>[14x]MAKELHFNKDMQALKRMQAGVDKLATVVGVTIGPKGRNVVLESKFGAPKIVNDGVTIAREVELSDPVENIGATLVRQAAARTNDTAGDGTTTATVLSAAFIAEGMKIVSAGTNPVQLVRGMEKTVQELVKELRKMSSVVQTDKDLANVACVSAGGNTDIGSLISDAMAKVGRTGVVTMEEGKTAEDQLVFVEGMQFERGYTSPYFVTDPERMICEYENCKILLVDKKISTARDIITILESAIRGNYPLLIMAEEVEQEALATLVVNKLRGTLKVVAIKAPGFGERRSSYLEDIAILTGGTV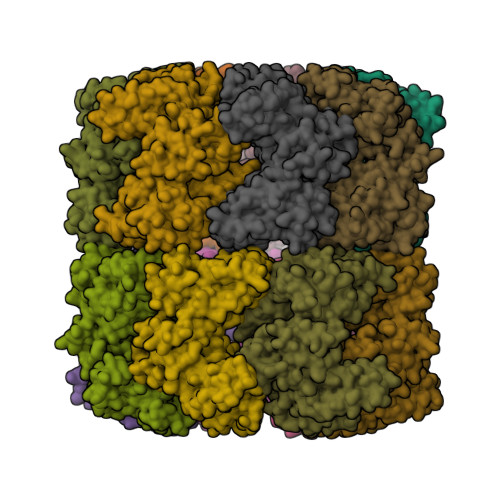VRDEMGVSLEQATDAVLGTAAKITITKERTTVVGDGSTAADVAARVKQIRNLQMQTDQDYEREKLQERIARLSGGVAIIQVGAQTETELKEKKLRVEDALNATRAAVEEGVVPGGGCTLLRLSEKVDVIKRRMTDPEQQMGADIIKRALCYPIKLIAQNAGVNGSVVMNEVMKNLDRPHYGYNAATDSFENLMETGIIDPSKVVRCSMENAVSVAKTFLLADVVVTELKEIEAGAKPNPVAPGAAGFGGGL>[2x]MGFLSGKRILVTGVASKLSIAYGIAQAMHREGAELA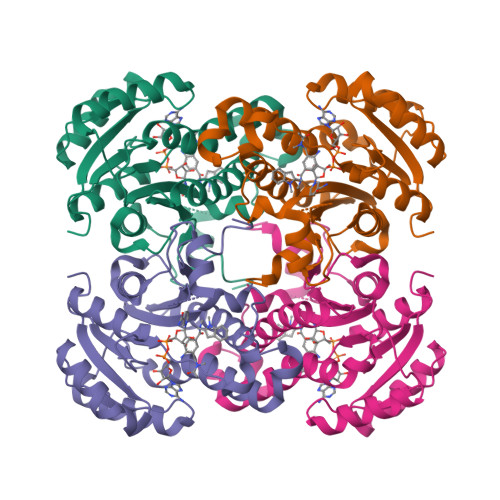FTYQNDKLKGRVEEFAAQLGSDIVLQCDVAEDASIDTMFAELGKVWPKFDGFVHSIGFAPGDQLDGDYVNAVTREGFKIAHDISSYSFVAMAKACRSMLNPGSALLTLSYLGAERAIPNYNVMGLAKASLEANVRYMANAMGPEGVRVNAISAGPIRTLAASGIKDFRKMLAHCEAVTPIRRTVTIEDVGNSAAFLCSDLSAGISGEVVHVDGGFSIAAMNELELK2-[5,6-BIS-(4-METHOXY-PHENYL)-FURO[2,3-D]PYRIMIDIN-4-YLAMINO]-ETHANOL 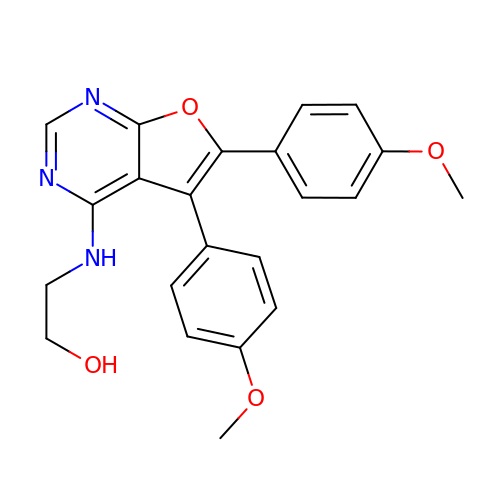| C22 H21 N3 O4 | ARBUGBBNEFAECO-UHFFFAOYSA-N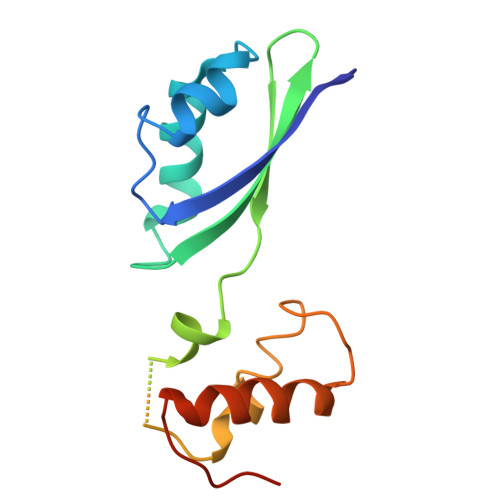> KKVVAVVKLQLPAGKATPAPPVGPALGQHGANIMEFVAAFNAATANMGDAIVPVEITIYADRSFTFVTKTPPASYLIRKAAGLEKGAHKPGREKVGRITWEQVLEIAKQKMPDLNTTDLEAAARMIAGSARSMGVEVVGAPEVKDA>[2x]MISKEYHIDEEVGFA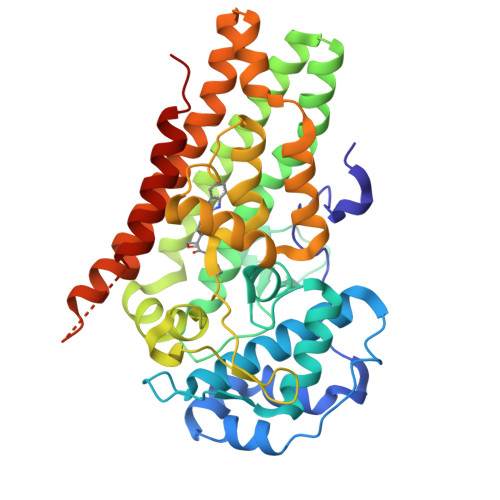LPNPQENLPDFYNDWMFIAKHLPDLIESGQLRERVEKLNMLSIDHLTDHKSQRLARLVLGCITMAYVWGKGHGDVRKVLPRNIAVPYCQLSKKLELPPILVYADCVLANWKKKDPNKPLTYENMDVLFSFRDGDCSKGFFLVSLLVEIAAASAIKVIPTVFKAMQMQERDTLLKALLEIASCLEKALQVFHQIHDHVNPKAFFSVLRIYLSGWKGNPQLSDGLVYEGFWEDPKEFAGGSAGQSSVFQCFDVLLGIQQTAGGGHAAQFLQDMRRYMPPAHRNFLCSLESNPSVREFVLSKGDAGLREAYDACVKALVSLRSYHLQIVTKYILIPASQQPKENKTSEDPSKLEAKGTGGTDLMNFLKTVRSTTEKSLLKEG> MPLILLPAVDVVEGRAVRLVQGKAGSQTEYGSAVDAALGWQRDGAEWIHLVDLDAAFGRGSNHELLAEVVGKLDVQVELSGGIRDDESLAAALATGCARVNVGTAALENPQWCARVIGEHGDQVAVGLDVQIIDGEHRLRGRGWETDGGDLW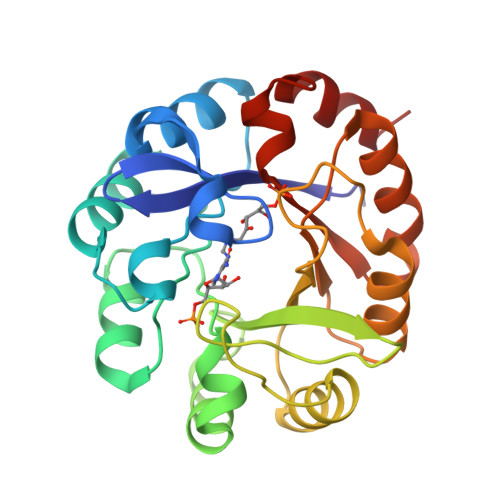DVLERLDSEGCSRFVVTDITKDGTLGGPNLDLLAGVADRTDAPVIASGGVSSLDDLRAIATLTHRGVEGAIVGKALYARRFTLPQALAAVRD> GAQVSRQNVGTHSTQNMVSNGSSLNYFNINYFKDAASSGASRL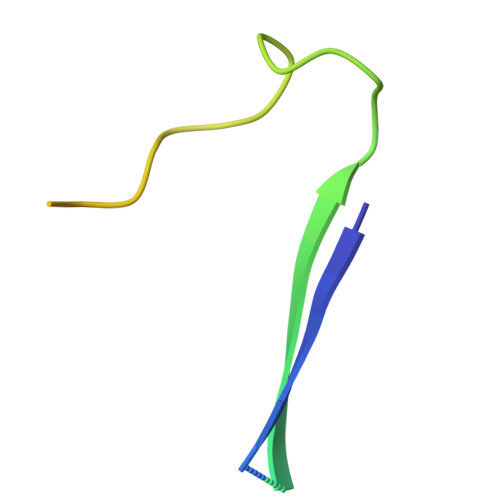DFSQDPSKFTDPVKDVLEKGIPTLQ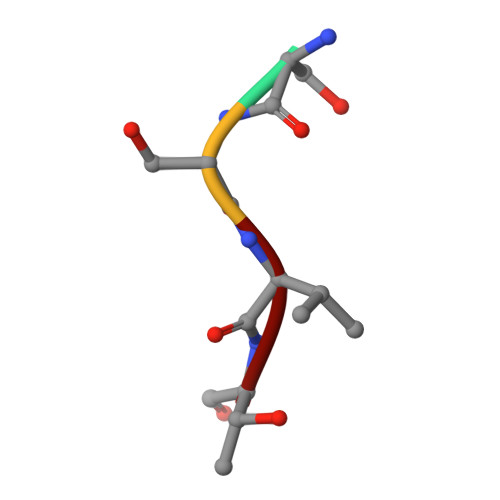> SSVT> DTTICEPFGTTTIQGRYVVQNNRWGSTAPQCVTATDTGFRVTQAD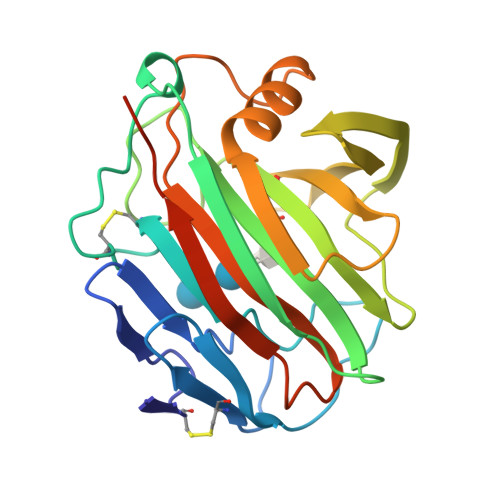GSAPTNGAPKSYPSVFNGCHYTNCSPGTDLPVRLDTVSAAPSSISYGFVDGAVYNASYDIWLDPTARTDGVNQTEIMIWFNRVGPIQPIGSPVGTASVGGRTWEVWSGGNGSNDVLSFVAPSAISGWSFDVMDFVRATVARGLAENDWYLTSVQAGFEPWQNGAGLAVNSFSSTVETGTPGGTDPGDPG>[5x]DSLKWIVFLLFLIVL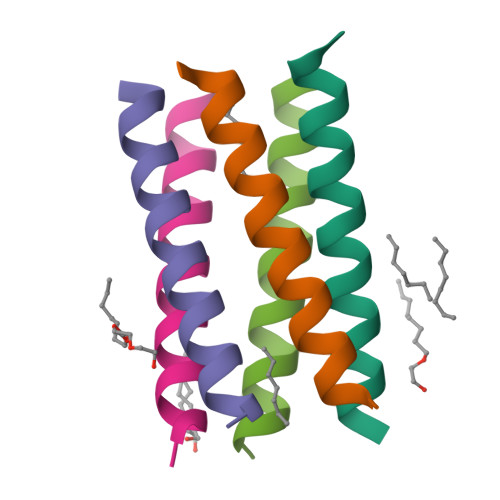LLLAIVFLLRGX> MLHTTRLWLGGYMMYHRKAMGTMKYSKWKGAHGGISHFYGRTPMVEEVRPNEPITLVDRRIMHYVHHSRLRHFQL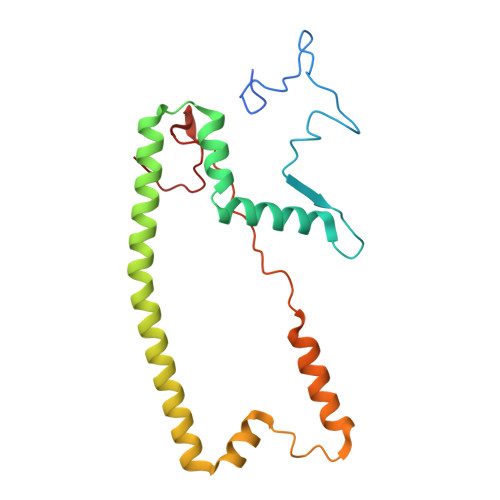FRSYQEKSNSTECKLREGEMLRRRWHRRLQKSFIAFMQFKTMKVLEDQARLVNTYGQAAVNAALGDPWNATDNVARERKSAAVRRQVRALPMVNVVPKHVATMKQIHNDRFNYRWRVN reserpine 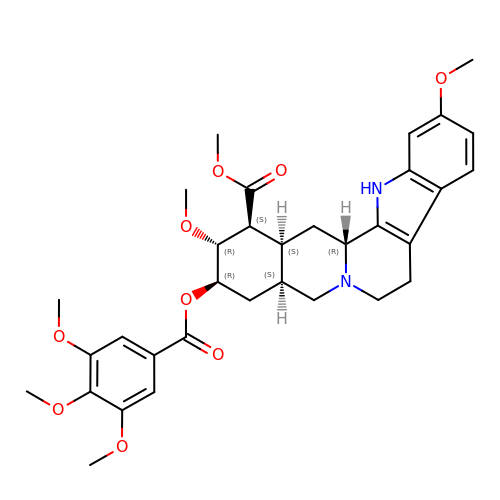| C33 H40 N2 O9 | QEVHRUUCFGRFIF-MDEJGZGSSA-N> PKVSVLITVTGVDQPGVTATLFEVLSRHGVEL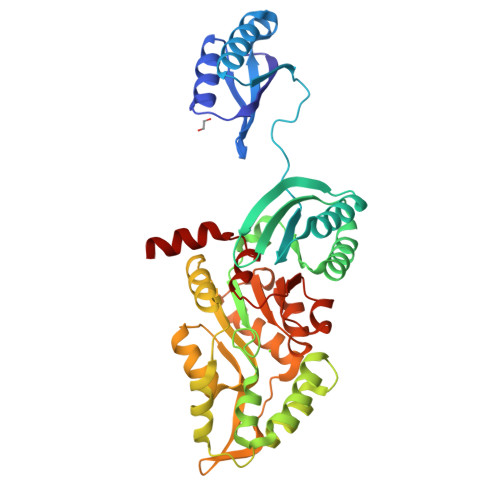LNVEQVVIRHRLTLGVLVCCPADVADGPALRHDVEAAIRKVGLDVSIERSDDVPIIREPSTHTIFVLGRPITAAAFGAVAREVAALGVNIDLIRGVSDYPVIGLELRVSVPPGADGALRTALNRVSSEEHVDVAVEDYTLERRAKRLIVFDVDSTLVQGEVIEMLAAKAGAEGQVAAITDAAMRGELDFAQSLQQRVATLAGLPATVIDEVAGQLELMPGARTTLRTLRRLGYACGVVAGGFARIIEPLAEELMLDYVAANELEIVDGTLTGRVVGPIIDRAGKATALREFAQRAGVPMAQTVAVGDGANDIDMLAAAGLGIAFNAKPALREVADASLSHPYLDTVLFLLGVTRGEIEAADAID> MADIYPLGKTHTEELNEIIVESAKEIAEPDTTMIQKLIDEHNPEPLLKGVRYYMCENDIEKKRRTYYDAAGQQLVDDTKTNNRTSHAWHKLFVDQKTQYLVGEPVTFTSDNKTLLEYVNELADDDFDDILNETVKNMSNKGIEYWHPFVDEEGEFDYVIFPAEEMIVVYKDNTRRDILFALRYYSYKGIMGEETQKAELYTDTHVYYYEKIDGVYQMDYSYGENNPRPHMTKGGQAIGWGRVPIIPFKNNEEMVSDLKFYKDLIDNYDSITSSTMDSFSDFQQIVYVLKNYDGENPKEFTANLRYHSVIKVSGDGGVDTLRAEIPVDSAAKELERIQDELYKSAQAVDNSPETIGGGATGPALEKLYALLDLKANMAERKIRAGLRLFFWFFAEYLRNTGKGDFNPDKELTMTFTRTRIQNDSEIVQSLVQGVTGGIM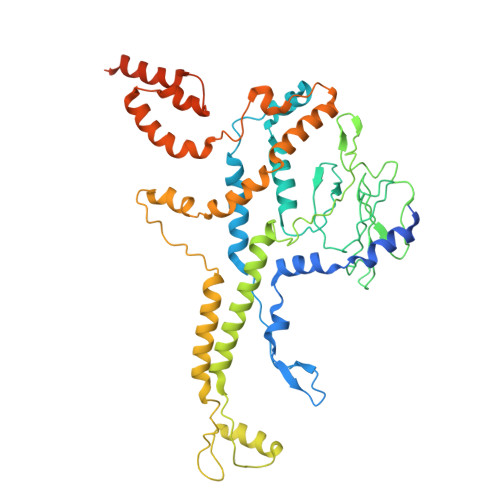SKETAVARNPFVQDPEEELARIEEEMNQYAEMQGNLLDDEGGDDDLEEDDPNAGAAESGGAGQVS> MANFLKNLHPLLRRDRNKKDNQDPNFALIDALNEEMNQVEKDAIESKLQSSLKTSTSEYLDKFGDWFGVYRKTDEKDDVYRARIIKYLLLKRGTNNAIIDAIKDYLGRDDIDVSVYEPFTNIFYTNKSHLNGEDHLMGYYYRFAVINVSIGDYFPVEIIDVINEFKPAGVTLYVTYDGASTIRGGAIIKWLDGLPKIETYQEFDRFTGYDDTFYGHINMNQSKDTDNSSSDIFKTNHSLINSLDVLTGSSSVGRQYINYGYVTSYVYNPGMTSSVNQISASTEGRGQEVPTDYYMYTSTKNNNTVELSMQTTSGVSYLYNN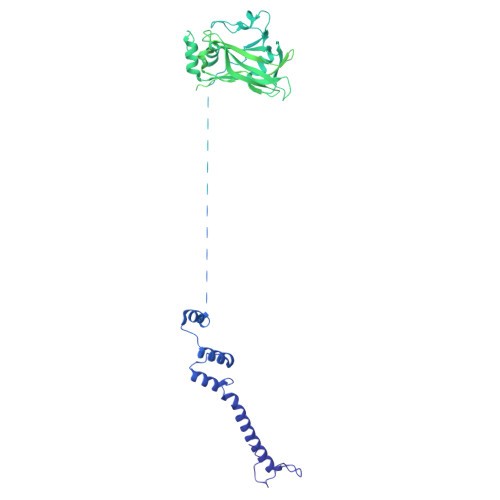FNFRDYMSKYRPQVDLQSDEARRIVSDYIKELSIDYYLSAVIPPDESIEIKLQVYDFSINRWLTVSINNLSFYEKNIGSNIGYIKDYLNSELNMFTRLEINAGKRDSVDIKVNYLDLMFYYYERGIYTIKPYKALIENYLDISRETYVEAFKIASLSNGDIITKTGFQPIGYLKLVGNYENTIPSTINIVAKDTDNNPIESNELDVYNTVENRNLLQSYKGVNTIAREITSTKEFTVSGWAKEIYSTNYLSKVLKPGKVYTLSFDMEITGNDPTLKSYSDNHGIYLYSNTKGIVVNGVKSMERTIGNKVSVTQTFTAPTITDHRLLIYTGRYTSDGKASTPPVFFNTVKITELKLTEGSSKLEYSPAPEDKPNVIEKGIKFNNILTNIQTLSINSDTILKNVTLYYSYYGDSWVELKTLGNISTGETTETNNLIDLYGLQTVDYSNINPMSKVSLRSIWNVKLGELNNQEGSLSNMPNDYFNAVWQDIDKLSDIELGSMRMVKDTEGGVFDGATGEIIKATLFNVGAYTDLDMLAYTLTNYTEPLTLGSSRLISELKEELLTSESFNVDNRIKVIDSIYEELPNTSIIKNGFVEREVTGSKYLDYGLYEPIEDGTRYKLIVEGEFKDNIEFISLYNSNPNFNETFIYPSEIINGVAEKEFIAKPSTEDKPRLNTDVRIYIRPYDSTISKVRRVELRKV Chitin is sensed in V. cholerae by the hybrid histidine kinase ChiS. In response to chitin, ChiS activates the expression of the chitin utilization program. In a recent study, we showed that unlike most histidine kinases, ChiS is capable of directly binding to DNA to regulate the expression of the chb operon. Previous work from our group demonstrated that ChiS is a noncanonical hybrid histidine kinase that contains a DBD at its C terminus.

Here, we present the crystal structure of the ChiS DBD at a resolution of 1.28 Å. Since no structures for close sequence homologs were available in the Protein Data Bank (PDB) to serve as search models for molecular replacement, we used the single-wavelength anomalous dispersion (SAD) technique to determine initial phases. The crystal diffracted to 1.28 Å resolution and belonged to the orthogonal C2221 space group with unit cell parameters of a = 51.91 Å, b = 78.61 Å, c = 72.37 Å, and α = β = γ = 90.00°. The structure includes 105 of 106 residues of the protein (1024 to 1128), two uncleavable residues of the purification tag, four sulfate ions (SO42−), one 2-(2-hydroxyethyloxy)ethanol molecule (PEG), two formic acid molecules (FMT), and 200 water molecules (HOH). The structure of the ChiS DBD revealed that it contains a fold that is reminiscent of the canonical helix-turn-helix (HTH) used by diverse DNA-binding proteins. Notably, however, the ChiS HTH has an insertion containing two anti-parallel β-strands connected by a turn between helix 2 and helix 3 that form a β-sheet. Structural insertion between these helices is not typical; thus, the sheet feature found here is a distinct variant of the HTH which we refer to as a helix-sheet-helix. Consistent with this idea, the β-sheet insertion has the highest B factor (a measure of structural motion) in the ChiS DBD structure, indicating that it is relatively flexible. Mapping these residues onto the ChiS DBD structure revealed that all five residues were found within the trihelical bundle that forms the helix-sheet-helix, which is consistent with this domain playing a critical role in DNA binding. Specifically, these residues were located in the β-sheet of the helix-sheet-helix (R1068), helix 3 (R1074, K1078), and helix 1 (R1090, R1092).

> GSSKQDLMRAVLVEAMTSALNYWERVSGQSKFTFAEQSGLWRVYLDRSTLQTRTLDKYLRIETLPKTPRWRTVLNSLDYILEHCKEAGPERTHIEMQRDKLQKLLTSE>RVCESQSHKFEGA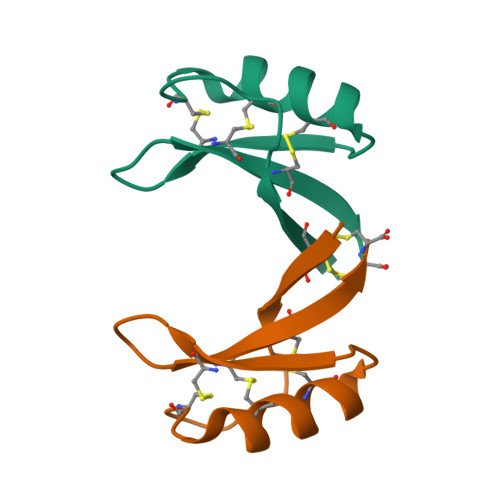CMGDHNCALVCRNEGFSGGKCKGLRRRCFCTKLC[2x]>GPHMTSDPVRQYLHEIGQVPLLTLEEEIDLARKVEEGMEAIKKLSEATGLDQELIREVVRAKILGTARIQKIPGLKEKPDPKTVEEVDGKLKSLPKELKRYLHIAREGEAARQHLIEANLRLVVSIAKKYTGRGLSFLDLIQEGNQGLIRAV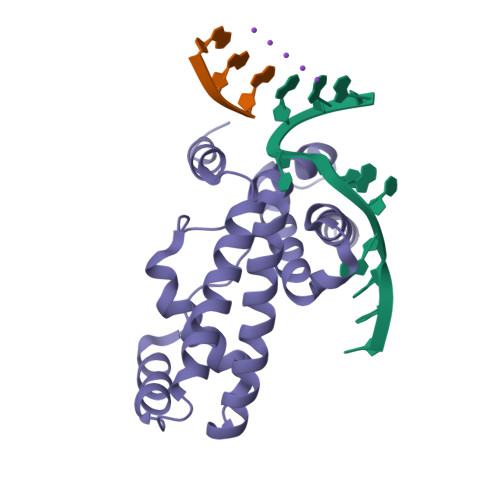EKFEYKRRFKFSTYATWWIRQAINRAIADQARTIRIPVHMVETINKLSRTARQLQQELGREPSYEEIAEAMGPGWDAKRVEETLKIAQEPVSL[2x]> DKKTEETTNIEDRIETTVVGATIINSQGSVGTTYCYSKPDGRPPSTVSDPVTRLGPTLSRHYTFKVGEWPH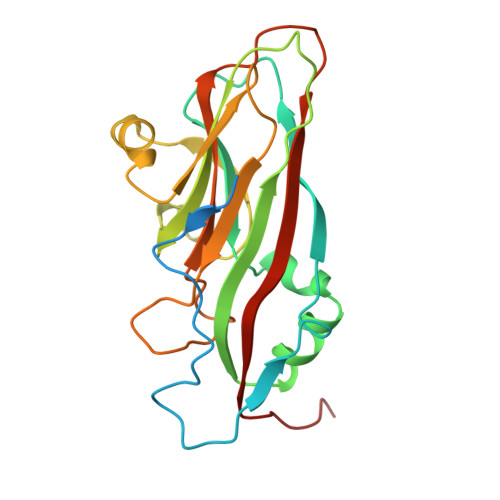SQSHGHAWICPLPSDKLKKMGSFHEVVKAHHLVKNGWDVVVQVNASFAHSGALCVAAVPEYEHTHEKALKWSELEEPAYTYQQLSVFPHQLLNLRTNSSVHLVMPYIGPGPTTNLTLHNPWTIVILILSELTGPGQTVPVTMSVAPIDAMVNGPLPNPE> GPGSEFCADQYWNEVAVIDAIPLAATEHDTMLEMSDMQVWSAGLTPSLVTAEDSGSLVPRGSGSKSDSNASFLRAARAGNLDKVVEYLKGGIDINTCNQNGLNALHLAAKEGHVGLVQELLGRGSSVDSATKKGNTALHIASLAGQAEVVKVLVKEGANINAQSQNGFTPLYMAAQENHIDVVKYLLENGANQSTATEDGFTPLAVALQQGHNQAVAILLENDTKGKVRLPALHIAARKDDTKSAALLLQNDHNADVQSKMMVNRTTESGFTPLHIAAHYGNVNVATLLLNRGAAVDFTARNGITPLHVASKRGNTNMVKLLLDRGGQIDAKTRDGLTPLHCAARSGHDQVVELLLERGAPLLARTKNGLSPLHMAAQGDHVECVKHLLQHKAPVDDVTLDYLTALHVAAHCGHYRVTKLLLDKRANPNARALNGFTPLHIACKKNRIKVMELLVKYGASIQAITESGLTPIHVAAFMGHLNIVLLLLQNGASPDVTNIRGETALHMAARAGQVEVVRCLLRNGALVDARAREEQTPLHIASRLGKTEIVQLLLQHMAHPDAATTNGYTPLHISAREGQVDVASVLLEAGAAHSLATKKGFTPLHVAAKY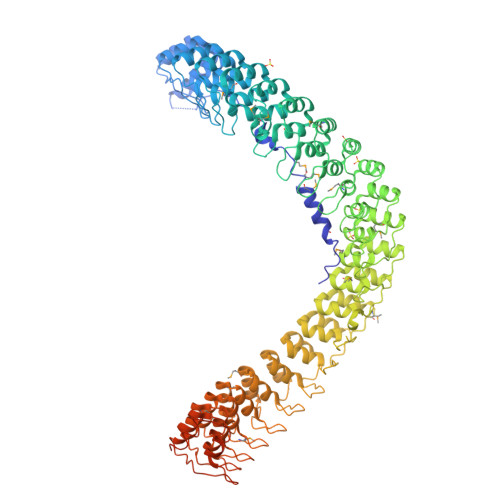GSLDVAKLLLQRRAAADSAGKNGLTPLHVAAHYDNQKVALLLLEKGASPHATAKNGYTPLHIAAKKNQMQIASTLLNYGAETNIVTKQGVTPLHLASQEGHTDMVTLLLDKGANIHMSTKSGLTSLHLAAQEDKVNVADILTKHGADQDAHTKLGYTPLIVACHYGNVKMVNFLLKQGANVNAKTKNGYTPLHQAAQQGHTHIINVLLQHGAKPNATTANGNTALAIAKRLGYISVVDTLKVVTEEVTTTTTTITEKHKLNVPETMTEVLDVSDEEGDDTMTGDGGEYLRPEDLKELGDD>GMKRKKKEEEEEKLIVTREFAKRWRDLSGQNHWKGMLQPLDQDLREYIIHYGEMAQAGYDTFNINTESQFAGASIYSRKDFFAKVGLEIAHPYTKYKVTKFIYATSDIHVPESFLLFPISREGWSKESNWMGYVAVTDDQGTALLGRRDIVVSWRGSVQPLEWVEDFEFGLVNAIKIFGERNDQVQIHQGWYSIYMSQDERSPFTKTNARDQVLREVGRLLEKYKDEEVSITICGHSLGAALATLSATDIVANGYNRPKSRPDKSCPVTAFVFASPRVGDSDFRKLFSGLEDIRVLRTRNLPDVIPIYPPIGYSEVGDEFPIDTRKSPYMKSPGNLATFHCLEGYLHGVAGTQGTNKADLFRLDVERAIGLVNKSVDGLKDECMVPGKWRVLKNKGMAQQDDGSWELVDHEIDDNEDLDF[2x]

The phospholipases are classified into four groups according to the cleavage site; phospholipase A1 (PLA1) cleaves sn-1 acyl chain, phospholipase A2 (PLA2) cleaves sn-2 acyl chain, phospholipase C (PLC) cleaves before the phosphate, and phospholipase D (PLD) cleaves after the phosphate. Here, we report the first molecular structures of plant PLA1s: AtDSEL and CaPLA1 derived from Arabidopsis thaliana and Capsicum annuum, respectively. AtDSEL and CaPLA1 are divided into the following two domains: the α/β hydrolase domain containing the lid domain, GXSXG motif, and catalytic triad and the C-terminal domain containing the dimerization domain. In addition to the conserved α/β hydrolase scaffold, GXSXG motif, and catalytic triad, plant PLA1s have an extended C-terminal domain composed of approximately 70 residues.

In Arabidopsis thaliana, DAD1 (At2g44810) was identified as an sn-1 specific acylhydrolase, and several studies have suggested that AtDSEL (Arabidopsis thaliana DAD1-like seedling establishment-related lipase), one of the homologues of DAD1, plays significant roles in the regulation of cellular processes such as seed germination, tissue growth, and seedling establishment. There are two AtDSEL molecules in the asymmetric unit, and each monomer chain consists of 16 α-helices (labeled α1–α16) and 11 β-strands (labeled β1–β11). AtDSEL shows the typical structure of an α/β hydrolase; core β-strands (β1–β3 and β6–β9) are flanked by several α-helices. An additional two β-strands (β4 and β5) and surrounding α-helices are also common in PLAs; however, C-terminal α-helices (α14–α16) and β-strands (β10 and β11), colored in blue, are unique features. AtDSEL has two disconnected loops caused by the disordered residues; Arg120 and Glu121 between β1 and β2 and from Pro159 to Leu160 between β3 and α5 could not be assigned due to the poor electron density map of the residues. The theoretical molecular weight of dimeric AtDSEL is 95.7 kDa, and calculated molecular weight from the AUC peak is 95.3 kDa, which strongly suggests that AtDSEL forms homodimers in solution. The dimerization domains of the AtDSEL homodimer cross each other and stretch in opposite directions. Met396 and Trp404 of one monomer and Trp388 of the other monomer interact with each other. The hydrophobic interactions are main driving force behind the formation of the dimerization of AtDSEL. AtDSEL specifically hydrolyzed the sn-1 acyl chain of 1,3-diacylglycerol (1,3-DAG) and 1-monoacylglycerol (1-MAG), suggesting that AtDSEL is an sn-1 specific lipase, as previously known.>[2x]MKQYLELMQKVLDEGTQKNDRTGTGTLSIFGHQMRFNLQDGFPLVTTQRCHLRSIIHELLWFLQGDTNIAYLHENNVTIWDEWADENGDLGPVYGKQWRAWPTPDGRHIDQITTVLNQLKNDPDSRRIIVSAWNVGELDKMALAPCHAFFQFYVADGKLSCQLYQRSCDVFLGLPFNIA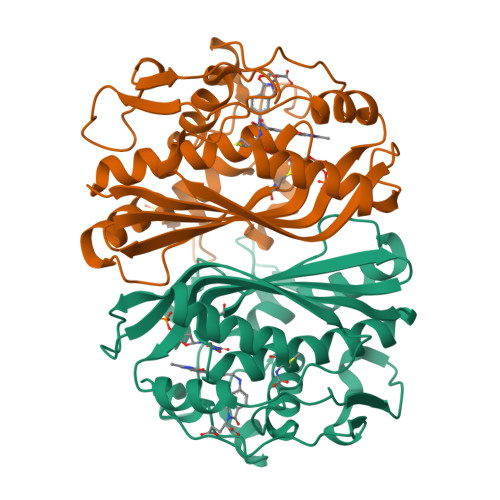SYALLVHMMAQQCDLEVGDFVWTGGDTHLYSNHMDQTHLQLSREPRPLPKLIIKRKPESIFDYRFEDFEIEGYDPHPGIKAPVAI>MGFDLDVEKKKENRNIPQANNLKIKVIGVGGAGNNAINRMIEIGIHGVEFVAVNTDLQVLEASNADVKI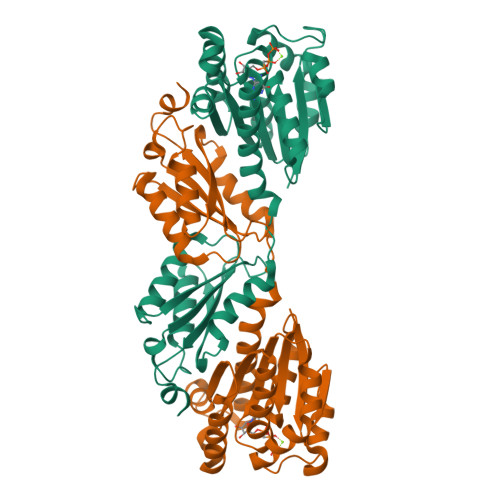QIGENITRGLGAGGRPEIGEQAALESEEKIREVLQDTHMVFITAGFGGGTGTGASPVIAKIAKEMGILTVAIVTTPFYFEGPERLKKAIEGLKKLRKHVDTLIKISNNKLMEELPRDVKIKDAFLKADETLHQGVKGISELITKRGYIRLTSRFARIESVMKDAGAAILGIGVGKGEHRAREAAKKAMESKLIEHPVENASSIVFNITAPSNIRMEEVHEAAMIIRQNSSEDADVKFGLIFDDEVPDDEIRVIFIATRFPDEDKILFPEGDIPAIYRYGLEGLL[2x]> MRGSHHHHHHGRSLNPLSTPQFDSTDETPASYNLAVRRAAPAVVNVYNRGLNTNSHNQLEIRTLGSGVIMDQRGYIITNKHVINDADQIIVALQDGRVFEALLVGSDSLTDLAVLKINATGGLPTIPINARRVPHIGDVVLAIGNPYNLGQTITQGIISATGRIGLNPTGRQNFLQTDASINPGNSGGALVNSLGELMGINTLSFDKSNDGETPEGIGF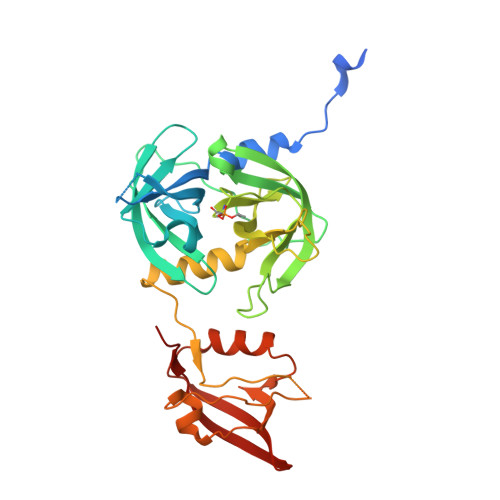AIPFQLATKIMDKLIRDGRVIRGYIGIGGREIAPLHAQGGGIDQLQGIVVNEVSPDGPAANAGIQVNDLIISVDNKPAISALETMAQVAEIRPGSVIPVVVMRDDKQLTLQVTIQEYPATN>MPATDTLSLSASEALARRRSVRAFTDRPVDRALLARIFEIAQRAPSGGNLQPWQATVVTGERWQAVQDAVAARIVMGREGFQPEYDIAPRGLTDPWDSRRFGVGEALYASLGIARDDKAGRIAQFQQNYRGFGAPVMLFLHCSRIMGPPQWADMGMWLQSVMLLLVEHGLASCPQECWAMYGATVRAELGLGDDQILFSGLAIGHADEEAPVNRWPVPRVGLDEVIDWQGFDA[2x]

Recently, the nitroreductase NfnB from Sphingopyxis sp. strain HMH exhibited metabolic activity for dinitroaniline herbicides including butralin and pendimethalin, triggering the initial steps of their degradation and detoxification. The homodimer NfnB is a member of the PnbA subgroup of the nitroreductase family. Each monomer displays a central α + β fold for the core domain, with a protruding middle region and an extended C-terminal region. The protruding middle region of Val75–Tyr129 represents a structural extension that is a common feature to members of the PnbA subgroup and functions as an opening wall connecting the coenzyme FMN-binding site to the surface, therefore serving as a substrate binding site.

Next, we determined the crystal structures of the two single mutants, Y88A and Y88F. Their structures were found to be nearly identical to the wildtype NfnB, with RMSD values of 0.38 Å for 428 Cα atoms in Y88A and 0.39 Å for 433 Cα atoms in Y88F. In the Y88F structure, the side chains of Phe88 and Arg100 are well ordered, at positions nearly identical to those of the wildtype NfnB. Compared with the wildtype NfnB, the side chain of Arg100 had been displaced by ∼4 Å toward the side chain of Asp97 near the entrance and was found within a ∼3-Å hydrogen-bonding distance from Asp97. Almost identical structural features of Arg100 were characterized in the Y88A mutant. Compared with the wildtype NfnB, the smaller side chain in Y88A and Y88F mutants exhibited a wider opening to the coenzyme FMN. The specific activity of the Y88A mutant toward butralin was ∼50% of the wildtype enzyme; its specific activities toward pendimethalin, oryzalin, and isopropalin were ∼42%, ∼42%, and ∼28%, respectively, of the wildtype NfnB for butralin. After comparing the efficiency of Y88A and Y88F, we concluded that both enzymes were more efficient than the wildtype NfnB, by about 2.3- and 3.1-fold, toward butralin, and by 11- and 30-fold against pendimethalin, respectively. In particular, Y88F exhibited higher efficiency toward butralin and pendimethalin, with a lower Km value than the wildtype NfnB, but Y88A was more competent than Y88F toward oryzalin and isopropalin, mainly because of its lower Km value. Consistent with the possible steric hindrance posed by Tyr88 in the wildtype NfnB, Y88F catalyzes enzyme reactions more efficiently for butralin and pendimethalin, and Y88A becomes competent for oryzalin and isopropalin, with larger hydrophobic substituents at the amino group.>[6x]TVYFHEEFKSMEHWTTSKHRDDFGKVEISAGKFYADAEKSKGLRLTEDARFYALSTAFPTPINNEKKSLVVSFSVKHEQDLKCGGGYIKLLPSMDPEKFHGETKYWLMFGPDRCGSQNRVHIILHYNGENREWSKRIRFPEDKLTHVYTLHIAADNSYEFFLDGESKAKGQLEEDWSLLLPREIVDGSGIPNPDFVEDSELHKVPEPLTHVGIDVWQVESGSIFKDIVIGDDLKE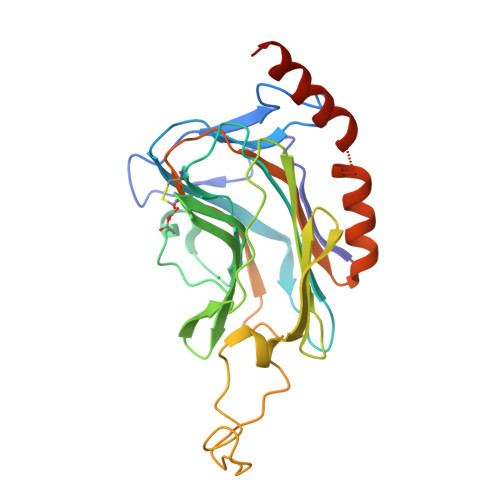VLDLVEKTYGGLKKAEADALKVMEDMEKGDHHHHHH>[2x]SNAMEQGMSKRILVPVAHGSEEMETVIIVDTLVRAGFQVTMAAVGDKLQVQGSRGVWLTAEQTLEACSA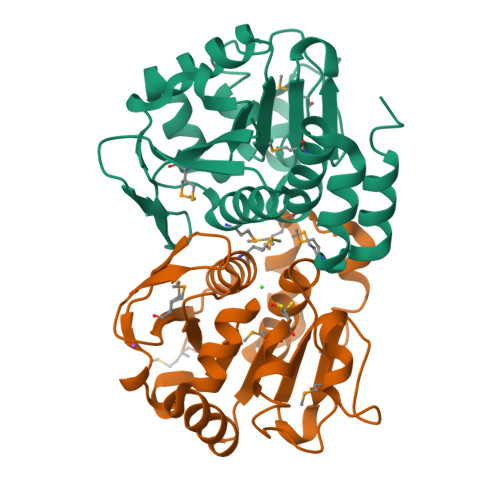EAFDALALPGGVGGAQAFADSTALLALIDAFSQQGKLVAAICATPALVFAKQQKFVGARMTCHPNFFDHIPSERLSRQRVCYYATQHLLTSQGPGTALEFALAMIALLAGVELAQHVAAPMVLHPQQLTELSGFIDAQS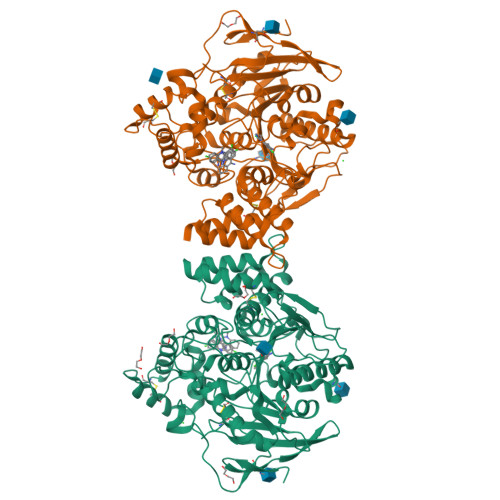>DDHSELLVNTKSGKVMGTRVPVLSSHISAFLGIPFAEPPVGNMRFRRPEPKKPWSGVWNASTYPNNCQQYVDEQFPGFSGSEMWNPNREMSEDCLYLNIWVPSPRPKSTTVMVWIYGGGFYSGSSTLDVYNGKYLAYTEEVVLVSLSYRVGAFGFLALHGSQEAPGNVGLLDQRMALQWVHDNIQFFGGDPKTVTIFGESAGGASVGMHILSPGSRDLFRRAILQSGSPNCPWASVSVAEGRRRAVELGRNLNCNLNSDEELIHCLREKKPQELIDVEWNVLPFDSIFRFSFVPVIDGEFFPTSLESMLNSGNFKKTQILLGVNKDEGSFFLLYGAPGFSKDSESKISREDFMSGVKLSVPHANDLGLDAVTLQYTDWMDDNNGIKNRDGLDDIVGDHNVICPLMHFVNKYTKFGNGTYLYFFNHRASNLVWPEWMGVIHGYEIEFVFGLPLVKELNYTAEEEALSRRIMHYWATFAKTGNPNEPHSQESKWPLFTTKEQKFIDLNTEPMKVHQRLRVQMCVFWNQFLPKLLNATACDGELSSSGTSSSKGIIFYVLFSILYLIF[2x]>GYV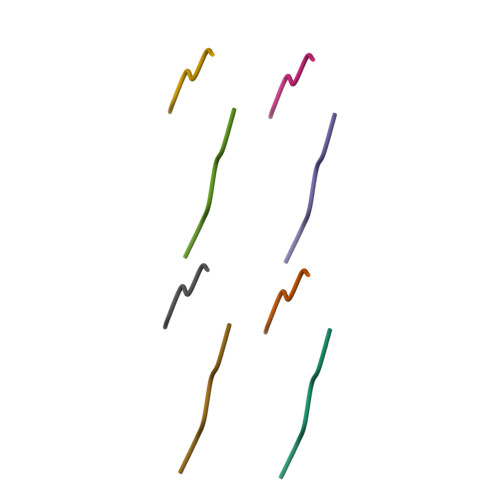LGS[2x]>EVILKDCSVPNPSWNKDLRLLFDQFMKKCEDGSWKRLPSYKRTPTEWIQDFKTHFLDPKLMKEEQMSQAQLFTRSFDDGLGFEYVMFYNDIEKRMVCLFQGGPYLEGPPGFIHGGAIATMIDATVGMCAMMAGGIVMTANLNINY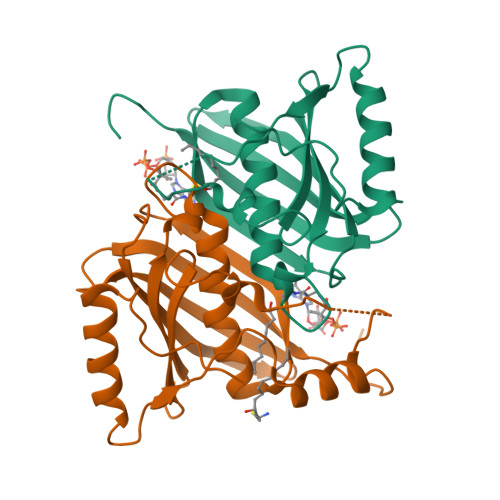KRPIPLCSVVMINSQLDKVEGRKFFVSCNVQSVDEKTLYSEATSLFIKLNPAKSLTLEHHHHHH[2x]>AWPEEKNYHQPAILNSSALRQIAEGTSISEMWQNDLQPLLIERYPGSPGSYAARQHIMQRIQRLQADWVLEIDTFLSQTPYGYRSFSNIISTLNPTAKRHLVLACHYDSKYFSHWNNRVFVGATDSAVPCAMMLELARALDKKLLSLKTVSDSKPDLSLQLIFFDGEEAFLHWSPQDSLYGSRHLAAKMASTPHPPGARGTSQLHGMDLLVLLDLIGAPNPTFPNFFPNSARWFERLQAIEHELHELGLLKDHSLEGRYFQNYSYGGVIQDDHIPFLRRGVPVLHL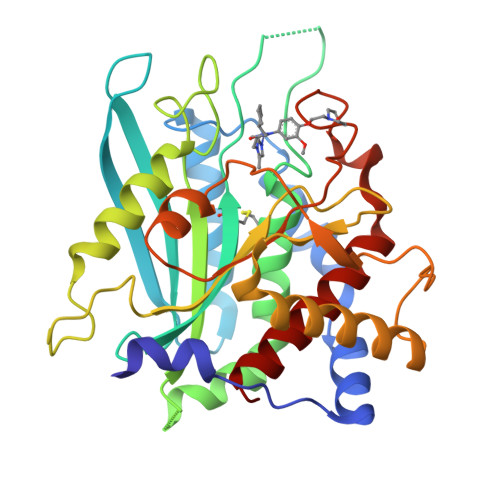IPSPFPEVWHTMDDNEENLDESTIDNLNKILQVFVLEYLHL[4x]O-METHYL-GLYCINE | C3 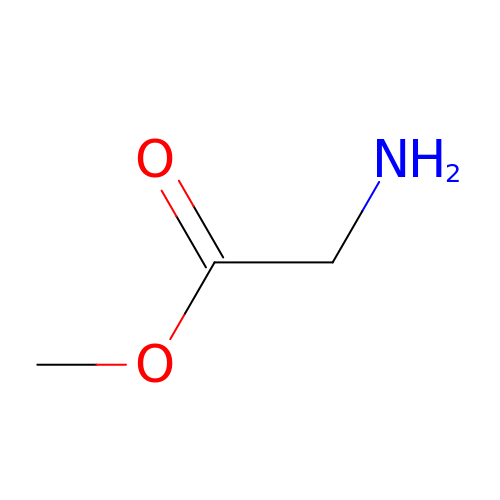H7 N O2 | KQSSATDQUYCRGS-UHFFFAOYSA-N>TSMDPSSPNYDKWEMERTDITMKHKLGGGQYGEVYEGVWKKYSLTVAVKTLKEDTMEVEEFLKEAAVMKEIKHPNLVQLLGVCTREPPFYIITEFMTYGNLLDYLRECNRQEVNAVVLLYMATQISSAMEYLEKKNFIHRDLAARNCLVGENHLVKVADFGLSRLMTGDTYTAHAGAKFPIKWTAPESLAYNKFSIKSDVWAFGVLLWEIATYGMSPYPGIDLSQVYELLEKDYRMERPEGCPEKVYELMRACWQWNPSDRPSFAEIHQAFET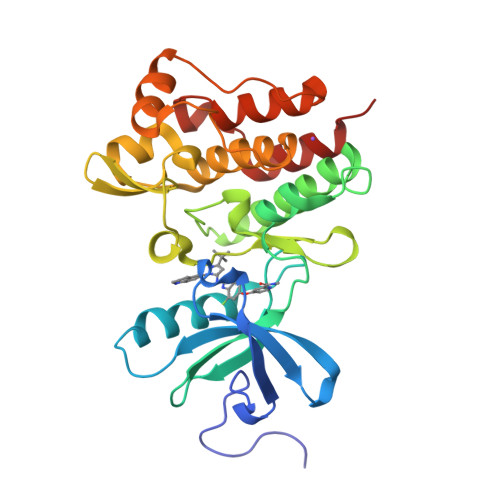MFQE[2x]> AAVT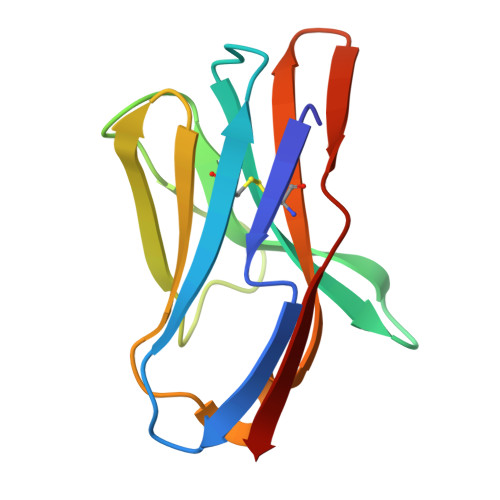QSPRNKVAVTGEKVTLSCQQTNNHNNMYWYRQDTGHGLRLIHYSYGAGSTEKGDIPDGYKASRPSQEQFSLILESATPSQTSVYFCASGGGGTLYFGAGTRLSVL>SNAMVLGKPQTDPTLEWFLSHCHIHKYPSKSTLIHQGEKAETLYYIVKGSVAVLIKDEEGKEMILSYLNQGDFIGELGLFEEGQERSAWVRAKTACEVAEISYKKFRQLIQVNPDILMRLSSQMANRLQITSEKVGNLAFLDVTGRIAQTLLNLAKQPDAMTHPDGMQIKITRQEIGQIVGCSRETVGRILKMLEDQNLISAHGKTIVVYGTR[2x]

Cyclic AMP (cAMP) receptor protein (Crp) is an important transcriptional regulator of Yersinia pestis. Crp is a 23.5-kDa transcriptional regulator that forms a dimer after binding its cAMP ligand. Dimerization allows activation or repression of gene expression by binding to the promoter region of its target genes. In turn, Crp regulates expression of the type III secretion system and the Pla protease essential for pneumonic plague.

Y. pestis Crp shares 99% sequence homology with Crp from E. coli, with differences located on the C helix at positions 119, 123, and 127. We considered that the sequence differences might affect cAMP binding or dimerization and thus cause changes in DNA binding. To investigate this, we carried out structural studies using protein crystallography and solved the crystal structure of Y. pestis Crp in complex with cAMP. Crp was crystallized as a dimer, and each monomer had cAMP bound to the binding site. The structures aligned closely, with root mean square deviation (RMSD) values of 0.8 Å for 185 pruned Cα atom pairs and 1.1 Å for all 200 pairs. Notably, in the Y. pestis structure, C helix residues S119, N123, and I127 (unlike S129 in the constitutive binding mutant of E. coli Crp) are directed away from cAMP, suggesting that these altered amino acids should not impact cAMP binding. The side chain of residue N123 is involved in dimer formation and directly interacts with the side chain of E78 from another chain. The N123 exchange for arginine, which occurs in Y. pestis, disrupts this interaction, but the S119 replacement for alanine restores the hydrogen bond to E78; thus, these two mutations do not alter the stability of the dimer. V127 in Crp from E. coli is pointed away from dimerization interface, and it is not involved in the cAMP binding, so isoleucine at this position in Y. pestis does not have any impact that contributes to binding of cAMP or to dimer formation. As confirmation of our findings, an electrophoretic mobility shift assay (EMSA) performed in the presence of cAMP indicated that Crp requires cAMP to bind a DNA fragment that corresponds to the pla promoter.>MRLELPVIPLRNTVILPHTTTPVDVGRAKSKRAVEEAMGADRLIFLVAQRDPEVDDPAPDDLYTWGVQAVVKQAMRLPDGTLQVMVEARARAQVTDYIPGPYLRARGEVFSEIFPIDEAVVRVLVEELKEAFEKYVANHKSLRLDRYQLEAVKGTSDPAMLADTIAYHATWTVAEKQEILELTDLEARLKKVLGLLSRDLERFELDKRVAQRVKEQMDTNQREYYLREQMKAIQKELGGEDGLSDLEALRKKIEEVGMPEAVKTKALKELDRLERMQQGSPEATVARTYLDWLTEVPWSKADPEVLDINHTRQVLDEDHYGLKDVKERILEYLAVRQLTQGLDVRNKAPILVLVGPPGVGKTSLGRSIARSMNRKFHRISLGGVRDEAEIRGHRRTYIGAMPGKLIHAMKQVGVINPVILLDEID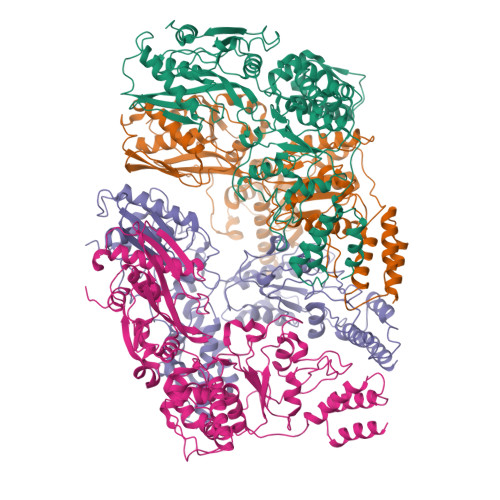KMSSDWRGDPASAMLEVLDPEQNNTFTDHYLDVPYDLSKVFFITTANTLQTIPRPLLDRMEVIEIPGYTNMEKQAIARQYLWPKQVRESGMEGRIEVTDAAILRVISEYTREAGVRGLERELGKIARKGAKFWLEGAWEGLRTIDASDIPTYLGIPRYRPDKAETEPQVGTAQGLAWTPVGGTLLTIEVAAVPGSGKLSLTGQLGEVMKESAQAALTYLRAHTQDYGLPEDFYNKVDLHVHVPDGATPKDGPSAGITMATAIASALSRRPARMDIAMTGEVSLRGKVMPIGGVKEKLLAAHQAGIHKIVLPKDNEAQLEELPKEVLEGLEIKLVEDVGEVLEYLLLPEPTMPPVVQPSDNRQQPGAGA[4x]>ETGETEPIVLEGKCLVVC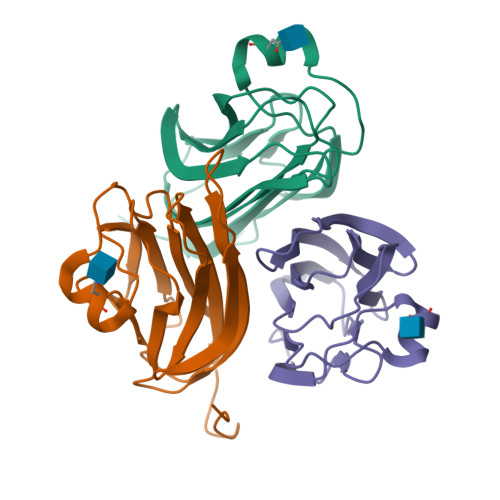DSNPTSDPTGTALGISSAKVAFSAIRSTNHEPSEMSNRTMIIYFDQVLVNIGNNFDSERSTFIAPRKGIYSFNFHVVKVYNRQTIQVSLMLNGWPVISAFAGDQDVTREAASNGVLIQMEKGDRAYLKLERGNLMGGWKYSTFSGFLVFPLGTKHHHHHH[3x]>MNSQLTLRALERGDLRFIHNLNNNRNIMSYWFEEPYESFDELEELYNKHIHDNAERRFVVEDAQKNLIGLVELIEINYIHRSAEFQIIIAPEHQGKGFARTLINRALDYSFTILNLHKIYLHVAVENPKAVHLYEECGFVEEGHLVEEGFINGRYQD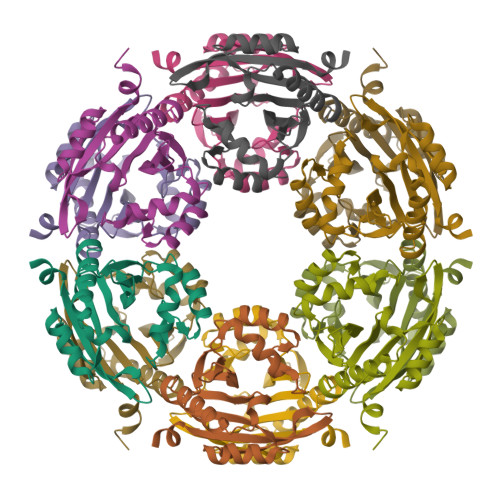VKRMYILQSKYLNRSE[3x]>APRKFFVGGNWKMNGDKKSLGELIHTLNGAKLSADTEVVCGAPSIYLDFARQKLDAKIGVAAQNCYKVPKGAFTGEISPAMIKDIGAAWVILGNPERRHVFGESDELIGQKVAHALAEGLGVIACIGEKLDEREAGITEKVVFEQTKAIADNVKDWSKVVLAYEPVWAIGTGKTATPQQAQEVHEKLRGWLKTHVSDAVAQSTRIIYGGSVTGGN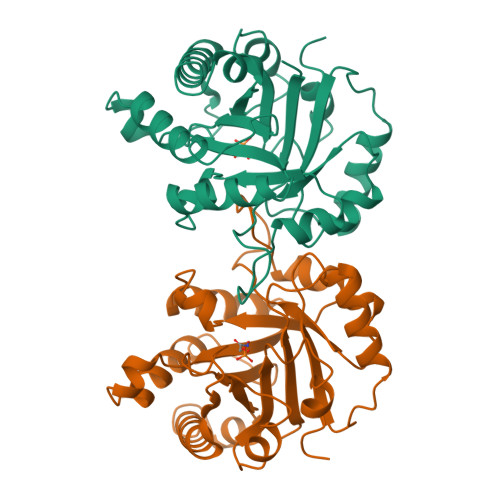CKELASQHDVDGFLVGGASLKPEFVDIINAKH[2x]>[6x]MSWSHPQFEKGAMTLSTIRWDVDIIAQSSIVHRDDYTSVGSDTFTLFRREKIIGPDGQILQIPLISGSSFRGVLRRVGEALTAEVLGYEDVALPVPAAHLLTNGGRLAKSAHPLTDEEERNLKELLPQIAVFGGAASGRVMSGLLSVSK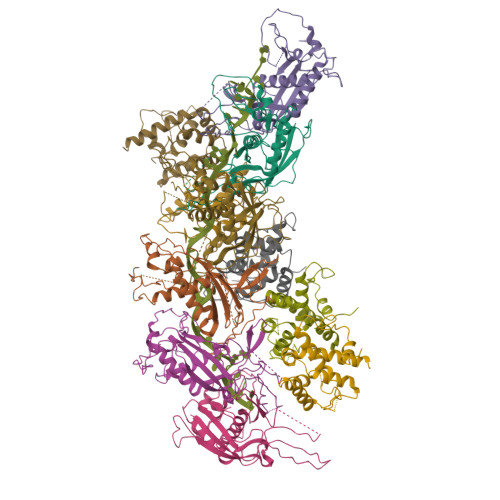VLPEIAELAHLLPRPPHSTPLLPAVLSVADESFTHLPDHRPSTGGAPRTDHADGSPLGRFAIETLPAGTRLQTWARLDNATEHQAAFFDNVLSTFAAHGHLGGRSAAGHGQVTATVTATALRGSLPRPTVDWVNQLADDRDAAIAALTRLT;>[5x]MTTPTPTQVWRATVPELPPLVDEAGDTGSATARAADTAERLLLLLHYSIDWESSWVADPKHRKTYWDELLPGRVRRAAYRADTLDRWWSEVAGQLGAPAPRHRDRRLELATLLREPALPVITVLRDSLPALLLRVRIIAEAVAAQRGNNSAATSSADPNEPA2-amino-6-[2-(1H-indol-6-yl)ethyl]pyrimidin-4(3H)-one | C14 H14 N4 O | 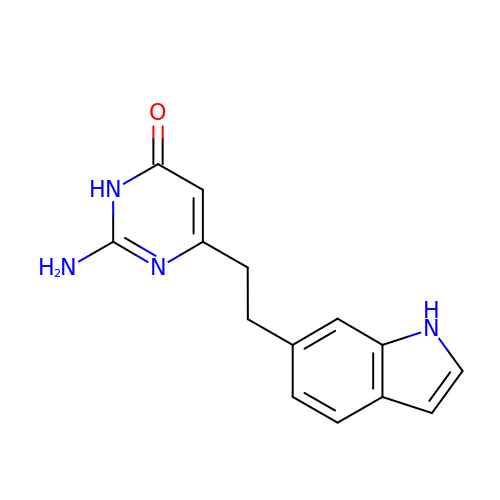VRAZIAJSKFRSIP-UHFFFAOYSA-N> SKSGVPRLLTASERERLEPFIDQIHYSPRYADDEYEYRHVMLPK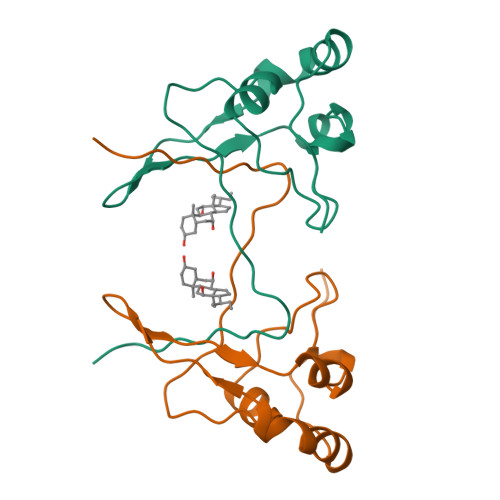AMLKAIPTDYFNPETGTLRILQEEEWRGLGITQSLGWEMYEVHVPEPHILLFKREKDYQMK> CCTAG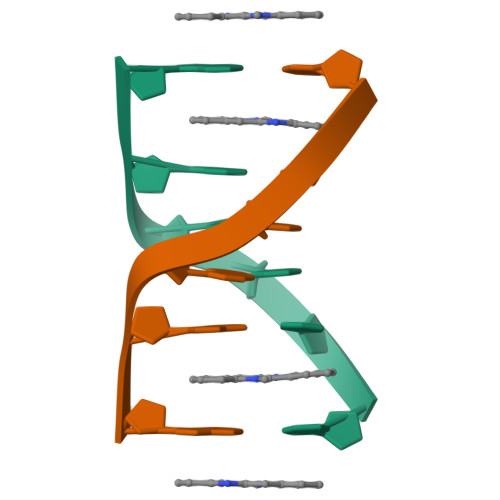G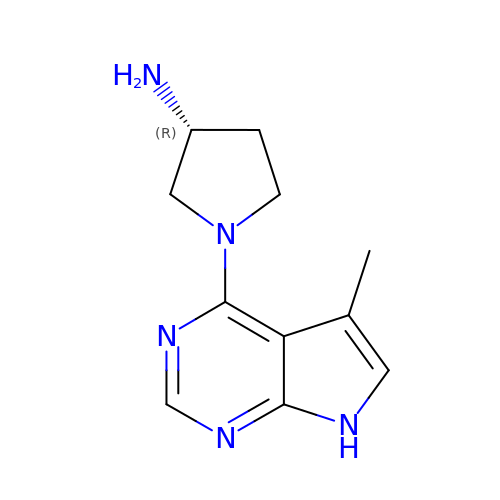(3R)-1-(5-methyl-7H-pyrrolo[2,3-d]pyrimidin-4-yl)pyrrolidin-3-amine | C11 H15 N5 | SMTIKTZYKPWXQP-MRVPVSSYSA-N> GAMGSELQSPEYKLSKLRTSTIMTDYNPNYCFAGKTSSISDLKEVPRKNITLIRGLGHGAFGEVYEGQVSGMPND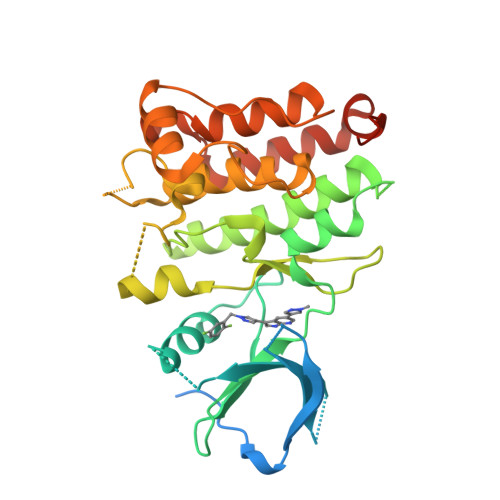PSPLQVAVKTLPEVCSEQDELDFLMEALIISKFNHQNIVRCIGVSLQSLPRFILLELMAGGDLKSFLRETRPRPSQPSSLAMLDLLHVARDIACGCQYLEENHFIHRDIAARNCLLTCPGPGRVAKIGDFGMARDIYRAGYYRKGGCAMLPVKWMPPEAFMEGIFTSKTDTWSFGVLLWEIFSLGYMPYPSKSNQEVLEFVTSGGRMDPPKNCPGPVYRIMTQCWQHQPEDRPNFAIILERIEYCTQDPDVINTALPIEYGPLVEEEEK> HHAADYVLYKDATKPVEDRVADLLGRMTLAEKIGQMTQIERLVATPDVLRDNFIGSLLSGGGSVPRKGATAKEWQDMVDGFQKACMSTRLGIPMIYGIDAVHGQNNVYGATIFPHNVGLGATRDPYLVKRIGEATALEVRATGIQYAFAPCIAVCRDPRWGRCYESYSEDRRIVQSMTELIPGLQGDVPKDFTSGMPFVAGKNKVAACAKHFVGDGGTVDGINENNTIINREGLMNIHMPAYKNAMDKGVSTVMISYSSWNGVKMHANQDLVTGYLKDTLKFKGFVISDWEGIDRITTPAGSDYSYSVKASILAGLDMIMVPNKYQQFISILTGHVNGGVIPMSRIDDAVTRILRVKFTMGLFENPYADPAMAEQLGKQEHRDLAREAARKSLVLLKNGKTSTDAPLLPLPKKAPKILVAGSHADNLGYQCGGWTIEFQGDTGRTTVGTTILEAVKAAVDPSTVVVFAENPDAEF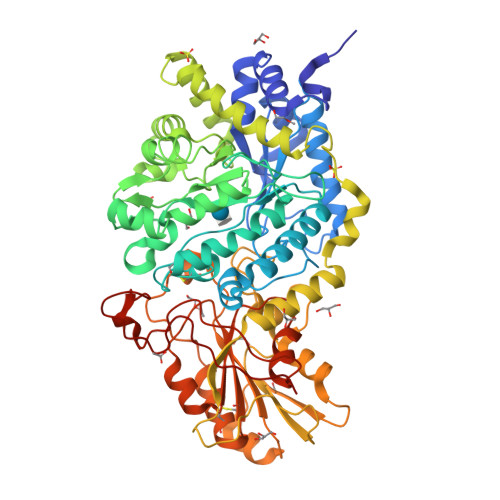VKSGGFSYAIVAVGEHPYTETKGDNLNLTIPEPGLSTVQAVCGGVRCATVLISGRPVVVQPLLAASDALVAAWLPGSEGQGVTDALFGDFGFTGRLPRTWFKSVDQLPMNVGDAHYDPLFRLGYGLTTNATKKY>GAMGWCIFIYNLGQDADEGILWQMFGPFGAVTNVKVIRDFNTNKCKGFGFVTMTNYEEAAMAIASLNGYRLGDKILQVSFKTNKSHK[3x]

HuR/ELAVL1 is an RNA-binding protein involved in differentiation and stress response that acts primarily by stabilizing messenger RNA (mRNA) targets. HuR specifically recognizes adenine and uridine-rich elements (ARE) and uridine-rich sequences in 3′ untranslated regions (3′UTRs) of mRNAs. Hu/ELAV proteins share a common protein architecture with two consecutive RRMs, separated from the third RRM (RRM3) by a less conserved, flexible hinge region of variable length. Here, we report crystal structures of HuR RRM3 free and bound to U- and AU-rich RNAs.

We initially selected two 6-mer RNA substrates: a sequence comprising the AUUUA pentamer derived from an ARE in TNF-α 3′UTR, (AU6tnf – UAUUUA), and a poly-U RNA that can be found in class III ARE elements without AUUUA repeats (U6 – UUUUUU). Both RNAs were bound by RRM3, with a Kd of 156 μM and 19 μM, respectively. We observed a substantial increase in RRM solubility after RNA binding and were thus able to use untagged RRM3 incubated with selected RNA ligands for structural studies of the complex. This allowed us to perform a comprehensive and comparative analysis of RRM3 interaction with three distinct RNA ligands: AUUUA motif-containing (AU6tnf), a U-rich motif with sparsely distributed adenosine residues (AU15) and a poly-U motif (U6). While in the structure of RRM3 with U6 and AU15, a uridine is recognized, in the case of AU6tnf RNA, an adenosine is bound in this pocket. In RRM3-AU6tnf and -AU15, the ribose in position 1 forms a (water-mediated) hydrogen bond with the main chain carbonyl of Lys285. On the 3′ end of the RNA, nucleotides in positions 5 and 6 are closer to the RRM3 β2β3 loop in case of the U6 ligand than when AU15 or AU6tnf are bound. In the case of AU6tnf, AU6 and GU6 the binding is predominantly in fast exchange, indicative of a weaker interaction. To summarize, the core of the RNA interactions with RRM3 is formed by three binding pockets with canonical aromatic residues from RNP2 and RNP1 (Phe247, Tyr249, Phe289) that recognize a U–U–U/A RNA sequence motif. The affected area correlates best with the dimeric interface found between chains A and B in the structures of RNA-bound RRM3 suggesting this is the dimerization interface in solution.1-(3-chloro-4-fluorophenyl)methanamine | C7 H7 Cl F N | 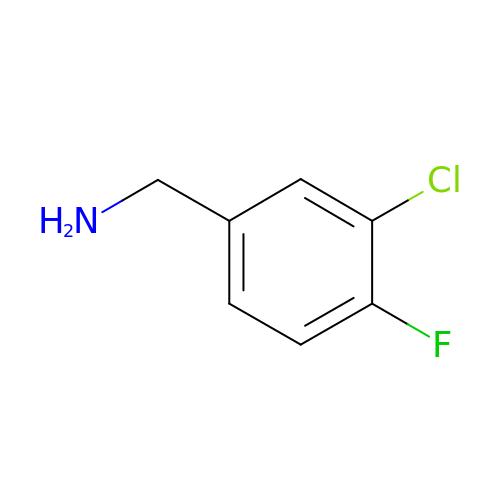LQAUXDMGRBWDIU-UHFFFAOYSA-N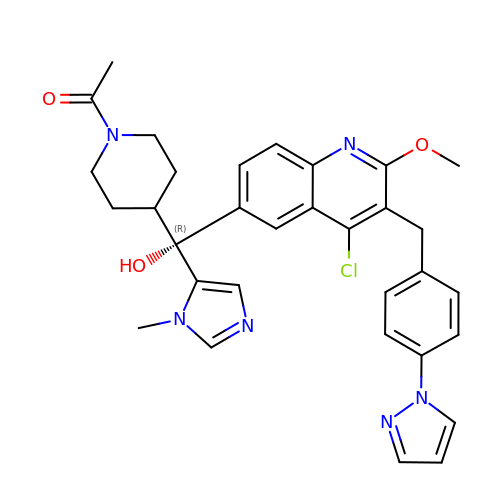1-{4-[(R)-(4-chloro-2-methoxy-3-{[4-(1H-pyrazol-1-yl)phenyl]methyl}quinolin-6-yl)(hydroxy)(1-methyl-1H-imidazol-5-yl)methyl]piperidin-1-yl}ethan-1-one | C32 H33 Cl N6 O3 | MAJOOHMQVBMIGI-JGCGQSQUSA-N>[2x]MAKK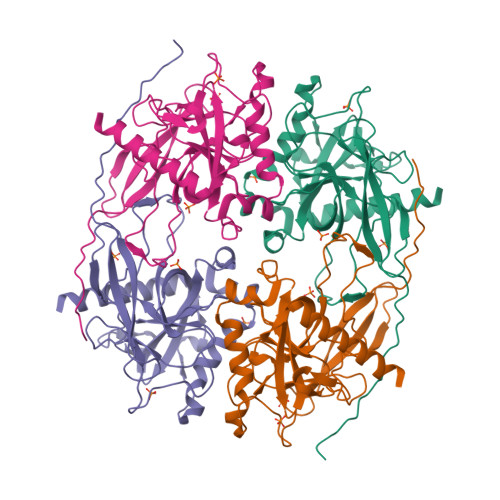DFFSMVSVDFAVPYHQQQLLTRETGELYTPSYRVLYYFRDMETGKELQVSPWHDIPLYVRDLVRTKPASLPMNRYNFICEIPKWTRAKFEIATGEPFNPIKQDIKNGVPRFYKHGDMMWNYGALPQTWESTDVVFEGGYVGDNDPIDAIEIGMTQFKVGQVGAVKVLGILGMIDDGQMDWKVICISHNDPICRFLKDIHDVPKFLPGCLDAIHEWFRVYKICQGGVENKFVFNGEFKDKSFAMKVIDESHYMWGNLRKI>GPHMSEAKAKAIGKVDDLLELYMGIRDIDLATTMFEAGKDKSNPDEFAVALDETLGDFAFPDEFLFDVWGAISDMKQGR[5x];>GPGSHDLSKWKYAELRDTINTSCDIELLAACREEFHRRLKVYHA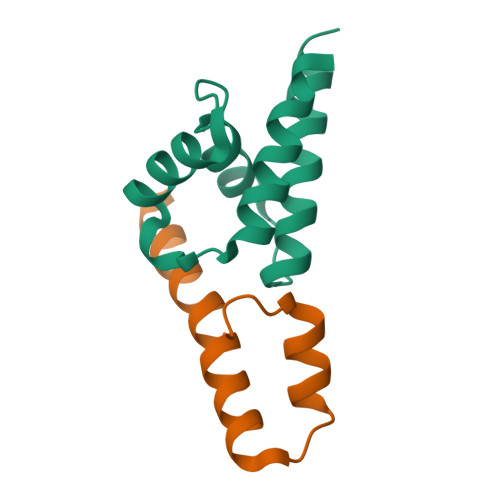WKSKN[5x]Influenza A virus has two surface glycoprotein antigens, hemagglutinin (HA) and neuraminidase (NA). NA is a homotetrameric type II transmembrane protein with an N-terminal cytoplasmic tail, a transmembrane domain, a hypervariable stalk region, and a C-terminal head domain. The head domain, which accounts for ~80% of NA protein sequence, contains an enzymatic active site that cleaves sialic acid to facilitate virus release and prevent virion aggregation. The enzymatic active site of influenza NA is also a target of several FDA-approved antivirals.

We aimed to analyze the fitness effects of mutations in the NA of H3N2 A/Moscow/10/1999 (Mos99) using deep mutational scanning. To further examine if the active site constrained the mutational tolerance of the surrounding residues, we determined the crystal structure of Mos99 NA in complex with sialic acid at 1.6 Å resolution. Although the sialidase enzymatic activity is the major function of NA, mutational tolerance and the distance from active site only showed weak correlation (Spearman’s rank correlation = 0.18). The correlation did not improve if we only included those residues within 15 Å from the active site (Spearman’s rank correlation = 0.03). These observations substantiate the notion that optimal enzymatic activity of NA relies on the global conformational stability of the tetramer. When we projected the mutational tolerance data on the structure, two clusters of solvent-exposed residues with low mutational tolerance were identified. The second cluster was at the membrane proximal side of the NA head domain, consisting of five residues with low mutational tolerance, namely R283, R288, D304, D355, and W383. Specifically, R283, R288, D304, and D355 form a network of electrostatic interactions. Furthermore, R288 forms π-stacking interactions with R283 and W383. As a result, the low mutational tolerance of these five residues is likely due to their critical role in NA folding stability.

> GSPSRAEYRNWSKPQCNITGFAPFSKDNSIRLSAGGDIWVTREPYVSCDPDKCYQFALGQGTTLNNGHSNDTVHDRTPYRTLLMNELGVPFHLGTKQVCIAWSSSSCHDGKAWLHVCVTGDDENATASFIYNGRLVDSIGSWSKKILRTQESECVCINGTCTVVMTDGSASGKADTKILFIEEGKIVHTSPLSGSAQHVEECSCYPRYPGVRCVCRDNWKGSNRPIVDINVKDYSIVSSYVCSGLVGDTPRKNDSSSSSHCLDPNNEEGGHGVKGWAFDDGNDVWMGRTISEKLRSGYETFKVIEGWSKPNSKLQINRQVIVDRGNRSGYSGIFSVEGKSCINRCFYVELIRGRKQETEVLWTSNSIVVFCGTSGTYGTGSWPDGADINLMPI heptyl 3-deoxy-alpha-D-mannopyranoside | C13 H26 O5 | 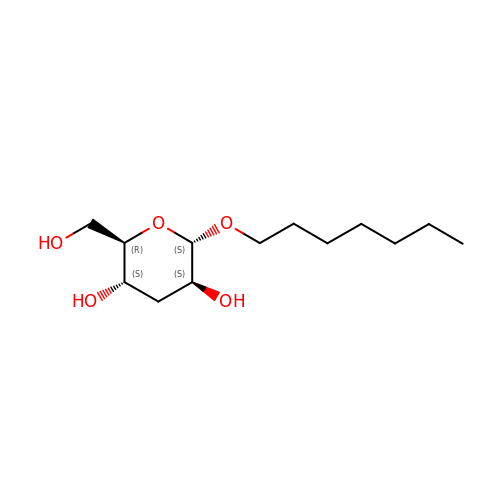PUHOACQHWFCDOT-RVMXOQNASA-N> MISVGSNSNAFKEAVKSVKTILRNLTDGEITISAYDTAWVALIDAGDKTPAFPSAVKWIAENQLSDGSWGDAYLFSYHDRLINTLACVVALRSWNLFPHQCNKGITFFRENIGKLEDENDEHMPIGFEVAFPSLLEIARGINIDVPYDSPVLKDIYAKKELKLTRIPKEIMHKIPTTLLHSLEGMRDLDWEKLLKLQSQDGSFLFSPSSTAFAFMQTRDSNCLEYLRNAVKRFNGGVPNVFPVDLFEHIWIVDRLQRLGISRYFEEEIKECLDYVHRYWTDNGICWARCSHVQDIDDTAMAFRLLRQHGYQVSADVFKNFEKEGEFFCFVGQSNQAVTGMFNLYRASQLAFPREEILKNAKEFSYNYLLEKREREELIDKWIIMKDLPGEIGFALEIPWYASLPRVETRFYIDQYGGENDVWIGKTLYRMPYVNNNGYLELAKQDYNNCQAQHQLEWDIFQKWYEENRLSEWGVRRSELLECYYLAAATIFESERSHERMVWAKSSVLVKAISSSFGESSDSRRSFSDQFHEYIANARRSDHHFNDRNMRLDRPGSVQASRLAGVLIGTLNQMSFDLFMSHGRDVNNLLYLSWGDWMEKWKLYGDEGEGELMVKMIILMKNNDLTNFFTHTHFVRLAEIINRICLPRQYLKARRNDEKEKTIKSMEKEMGKMVELAL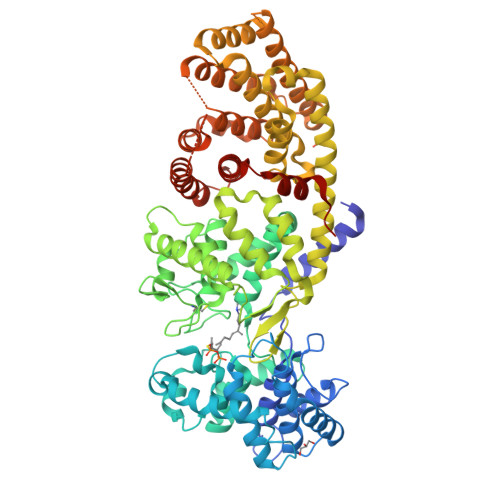SESDTFRDVSITFLDVAKAFYYFALCGDHLQTHISKVLFQKVGSHHHHHH>[4x]MNGERIIAFQGRPGAYSDLACRQARPGWTTLPCQTFAQTIAAVHDGRAELAMLACENSLAGRVPDIHALLPEAGLFIVGEHFQRVEHCLLGIPGSTLADARRIHTHPVAMAQVRGIITELGLDPVVEFDTAGAAEMVREWGRKEDVAVASALAAELNGLEILRRNVEDATHNTTRFYIASRRPATLPPPGPGFMTTLLFRVNNQPGALYKALGGLATAGVNMTRLESYMLEGSFSATQFLMDVEGHPEAPPLARALDELSFFSEQQEILGVYPASPFRRKP

GqqA strongly interfered with N-acyl-homoserine lactone (AHL) quorum sensing signals from Gram-negative bacteria and affected biofilm formation in its native host strain Komagataeibacter europaeus. ESI–MS–MS data showed unambiguously that GqqA hydrolyzes the amide bond of the acyl side-chain of AHL molecules, but not the lactone ring. Consistent with this observation the protein sequence does not carry a conserved Zn2+ binding motif, known to be essential for metal-dependent lactonases, but in fact harboring the typical periplasmatic binding protein domain (PBP domain), acting as catalytic domain. Structural data together with a phylogenetic analysis and the enzymatic characteristics implied that GqqA represents the first example of a till now unknown, third and novel subclass of acylases.

We solved and refined the native GqqA three-dimensional structure to 2.5 Å resolution, utilizing SAD phases obtained from a truncated and Se modified version of GqqA. DLS and SAXS measurements indicated a GqqA dimer in solution, which is also present in the crystal structure with a rather extended interface area of approx. 2230 Å2 between the monomers. A GqqA monomer itself consists of three domains. The N-terminal and middle domain of GqqA consist of a mixed five-stranded β-sheet with three parallel strands, surrounded by three α-helices. The C-terminal ACT domain is formed by a four-stranded anti-parallel β-sheet and two helices. The symmetry related mate of the ACT domain complements an extended central β-sheet structure of the functional homodimer. In the C-terminal regions of both monomers within the dimer interface we identified two L-Phe molecules. The PBP domain is folded into two structurally similar subdomains which form a cleft for the putative active site. Docking studies applying the native GqqA structure and the potential substrate N-octanoyl-L-homoserine lactone suggest that the lactone ring most probably binds to the polar residues Y16, S17 and T174 located in the cleft typical for the subdomains of PDT. According to this data the GqqA crystal structure we analysed corresponds to a closed conformation.>PSVYDAAAQLTADVKKDLRDSWKVIGSDKKGNGVA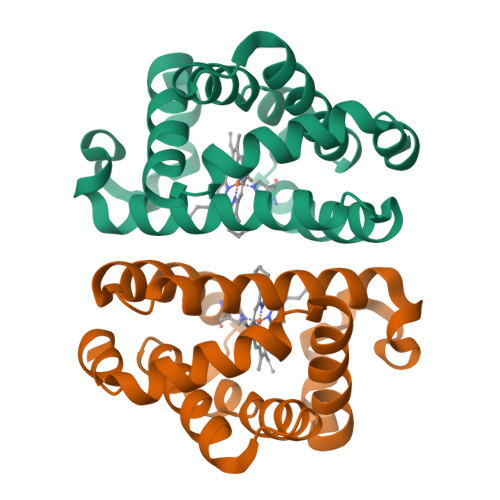LMTTLFADNQETIGYFKRLGNVSQGMANDKLRGHSITLMYALQNFIDQLDNPDDLVCVVEKFAVNHITRKISAAEFGKINGPIKKVLASKNFGDKYANAWAKLVAVVQAAL[4x]> GSHMVQLVNFLQSEHPQTIAVVLSYLDPPVAAQILGAL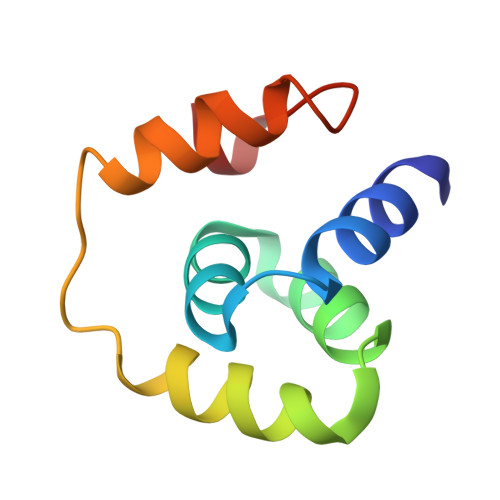PEELQTEVLKRIALLERTSPEVVKEIERNLEKKISGFSRTFS N-[2-(2,6-dichlorophenyl)-1H-imidazo[4,5-c]pyridin-4-yl]cyclopropanecarboxamide | C16 H12 Cl2 N4 O | 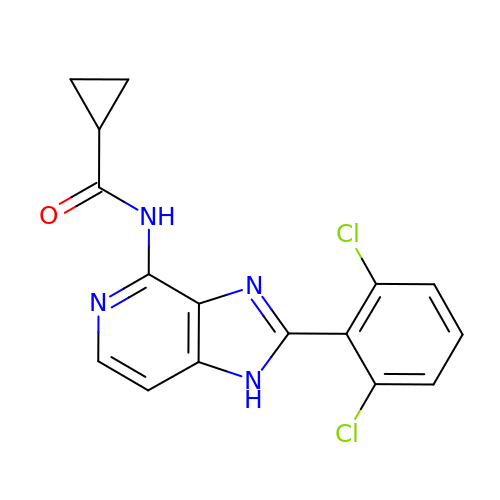OFPQQEBBZKPLFE-UHFFFAOYSA-N> RSYGTPELDEDDLEAELDALGDELL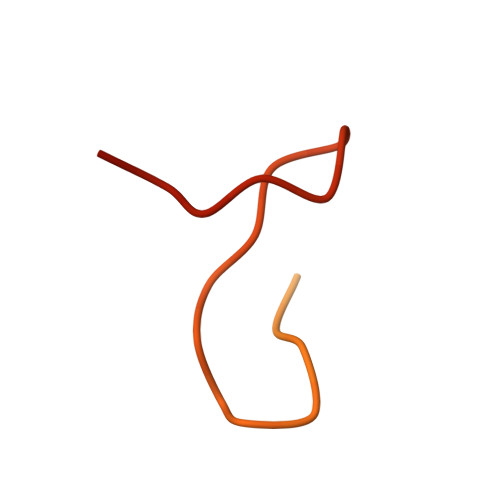ADEDSSYLDEAASAPAIPEGVPTDTKNKDGVLVDEFGLPQIPAS> AQDDYRYIHFLTQHYDAKPKGRNDEYCFNMM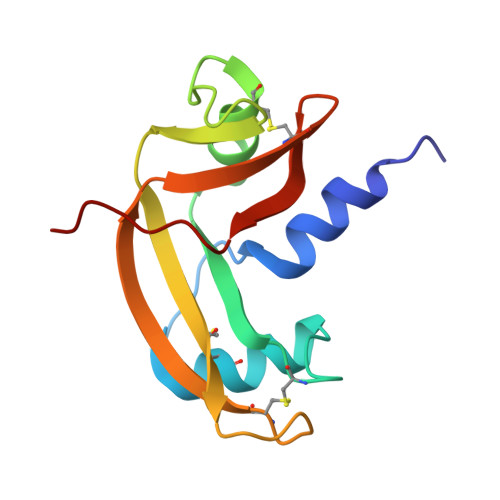KNRRLTRPCKDRNTFIHGNKNDIKAICEDRNGQPYRGDLRISKSEFQITICKHKGGSSRPPCRYGATEDSRVIVVGCENGLPVHFDESFITPRH>[2x]AYTTFSATKNDQLKEPMFFGQPVQVARYDQQKYDIFEKLIEKQLSFFWRPEEVDVSRDRIDYQALPEHEKHIFISNLKYQTLLDSIQGRSPNVALLPLISIPELETWVETWAFSETIHSRSYTHIIRNIVNDPSVVFDDIVTNEQIQKRAEGISSYYDELIEMTSYWHLLGEGTH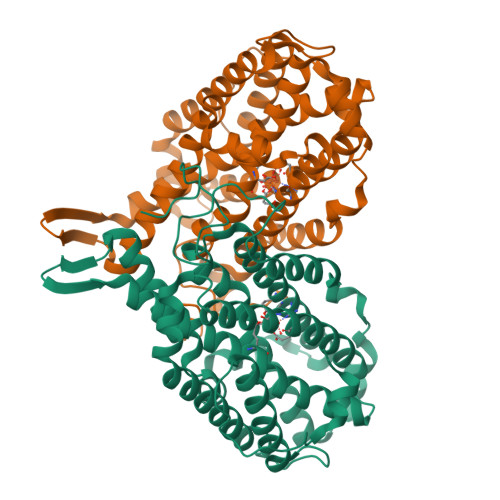TVNGKTVTVSLRELKKKLYLCLMSVNALEAIRFYVSFACSFAFAERELMEGNAKIIRLIARDEALHLTGTQHMLNLLRSGADDPEMAEIAEECKQECYDLFVQAAQQEKDWADYLFRDGSMIGLNKDILCQYVEYITNIRMQAVGLDLPFNTRSNPIPWINTWLVSDNVQVAPQEVEVSSYLVGQIDSEVDTDDLSNFQL6-chloranyl-5,7-dimethyl-4-(1~{H}-1,2,3,4-tetrazol-5-ylmethyl)-1,4-benzoxazin-3-one | C12 H12 Cl N5 O2 | 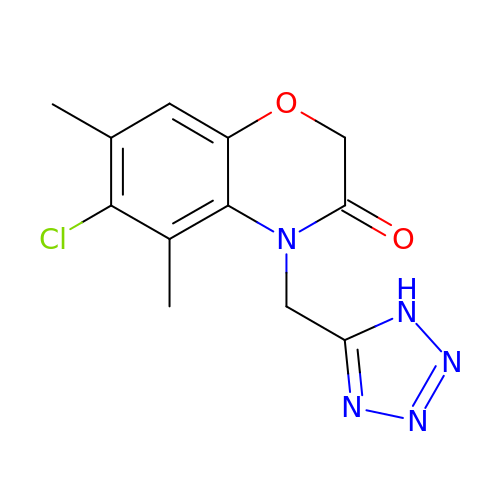YZYWMDSEBRUKPG-UHFFFAOYSA-N>[2x]GSFTMDFPYDLNALFPERISVLDSNLSAGRKAH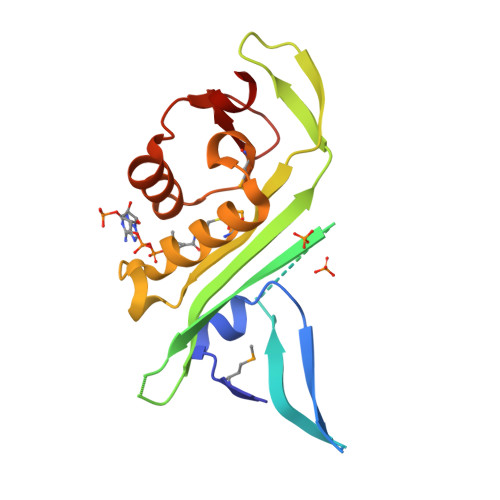GRPDPLPQVTTVIDELGKASSKAQQLPAPITSAAKLQANRHHLYLLKDGEQNGGRGVIVGFLKVGYKKLFLLDQRGAHLETEPLCVLDFYVTETLQRHGYGSELFDFMLKHKQVEPAQMAYDRPSPKFLSFLEKRYDLRNSVPQVNNFVVFAGFFQS> QDADKLPHTKVTLVAPPQVHPHEQASKTGPKVVEFTMTIEEKKMVIDDKGTTLQAMTFNGSMPGPTLVVHEGDYVQLTLVNPATNAMPHNVDFHGATGALGGAKLTNVNPGEQATLRFKADRSGTFVYHCAPEGMVPWHVVSGQSGTLMVLPRDGLKDPEGKPLHYDRAYTIGEFDLYIPKGPDGKYKDYATLAESYGDTVQVMRTL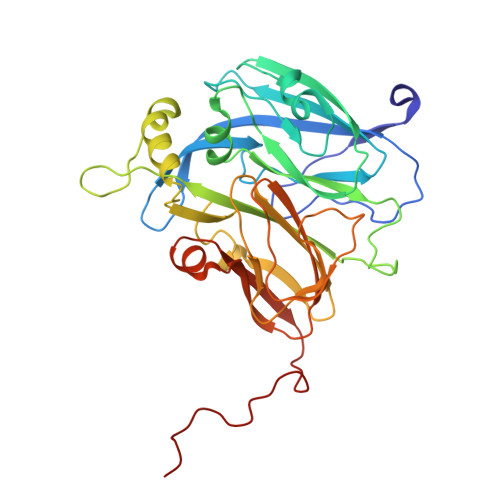TPSHIVFNGKVGALTGANALTAKVGETVLLIHSQANRDTRPHLIGGHGDWVWETGKFANPPQRDLETWFIRGGSAGAALYTFKQPGVYAYLNHNLIEAFELGAAGHIKVEGKWNDDLMKQIKAPAPIPR In this study, we describe the structure and function of a highly specific ion channel blocker from the salivary gland of X. cheopis, which belongs to the FS family and has been given the name FS50. The FS family of peptides is unique to fleas and has been identified from the salivary glands of the rat flea Xenopsylla cheopis (Rots) and the cat flea Ctenocephalides felis. FS proteins contain six to eight conserved cysteine residues forming three or four disulfide bonds and show relatively weak similarity to scorpion toxins. In this study we have shown that FS50, a salivary component of the rat flea, is a blocker of the sodium channel NaV1.5 that is capable of protecting rats and monkeys from barium chloride-induced arrhythmias.

FS50 contains a cysteine-stabilized core βαββ structure having a general similarity to that found in the scorpion β toxins. The protein also contains a second domain made up of a small βαβ structure that is connected to the core domain through a coil region. While a second domain (the NC-globule) found in scorpion β-toxins is made up of elements both N- and C-terminal to the core domain, the βαβ domain of FS50 is comprised only of a long N-terminal extension. The C-terminus is truncated after β-strand C of the core domain and does not contribute to the second domain. The core-domain of FS50 is composed of a five-turn α-helix (residues 37–52) packed against a three-stranded antiparallel β-sheet (residues 25–27, 55–59, and 72–75) and is stabilized by three disulfide bonds (Cys 44-Cys 72, Cys 48-Cys 74 and Cys 31-Cys 59). In the second domain, the α-helix and two-stranded antiparallel β-sheet are formed by residues 5–9, residues 1–3, and residues 17–21, respectively. A fourth disulfide bridge between Cys 7 and Cys 52 connects the two domains. Notably, the loop connecting β-strands 1 and 2 of the core domain is elongated and folded back over the core domain β-sheet. Along with the βαβ domain, this arrangement produces a somewhat flattened surface unlike the protruding C-terminal sequence seen in the scorpion toxins. From its structure, it would appear that the binding mode of FS50 is unlike that of the scorpion toxins, and outside of general similarities in their overall folds, the two types of proteins probably function differently.

>MWKVSERCLKGHGKFQADQEIGNGLATAKGQCKGTDSDQKKAGKCDKHCTGVCLGSGGSCGDGSSQKPNKEDCYCKSK[2x]> MNIVLMGLPGAGKGTQADRIVEKYGTPHISTGDMFRAAIQEGTELGVKAKSFMDQGALVPDEVTIGIVRERLSKSDCDNGFLLDGFPRTVPQAEALDQLLADMGRKIEHVLNIQ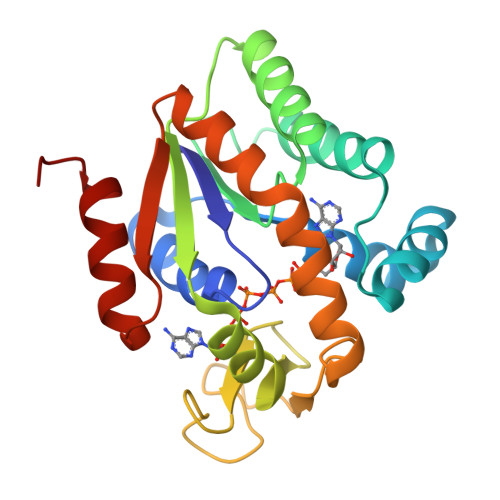VEKEELIARLTGRRICKVCGTSYHLLFNPPQVEGKCDKDGGELYQRADDNPDTVTNRLEVNMNQTAPLLAFYDSKEVLVNINGQKDIKDVFKDLDVILQGNGQ5'-{[(benzenecarbonyl)sulfamoyl]amino}-5'-deoxyadenosine 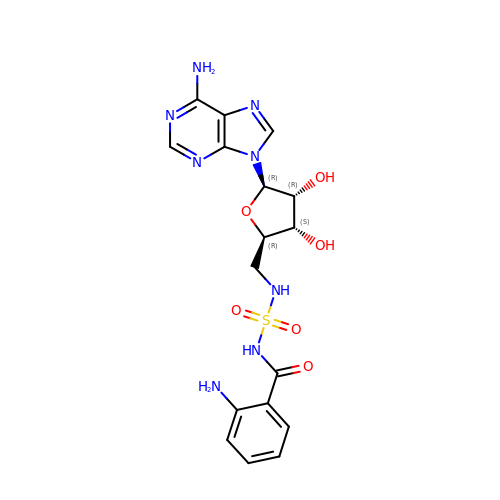| C17 H20 N8 O6 S | VRCFLQCMFIZPPZ-CNEMSGBDSA-N>AFEDRDPTQFEERHLKFLQQLGKGNFGSVEMCRYDPLQDNTGEVVAVKKLQHSTEEHLRDFEREIEILKSLQHDNIVKYKGVCYSAGRRNLKLIMEYLPYGSLRDYLQAHAERIDHIKLLQYTSQICKGMEYLGTKRYIHRDLATRNILVENENRVKIGDFGLTKVLPQDKEYYKVKEPGESPIFWYAPESLTESKFSVASDVWSFGVVLYELFTYIEKSKSPPAE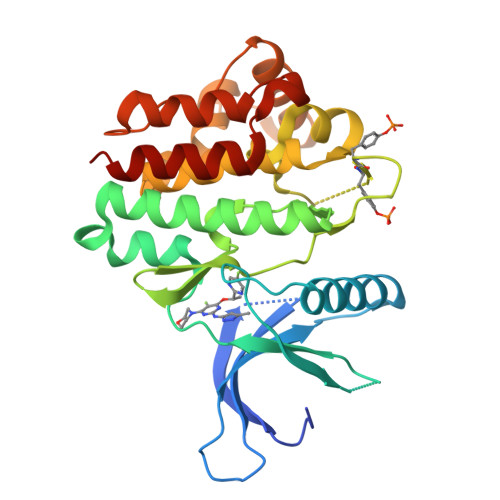FMRMIGNDKQGQMIVFHLIELLKNNGRLPRPDGCPDEIYMIMTECWNNNVNQRPSFRDLALRVDQIRDQMAG[2x]>[8x]MSLIVITGASSGLGAELAKLYDAEGKATYLTGRSESKLSTVTN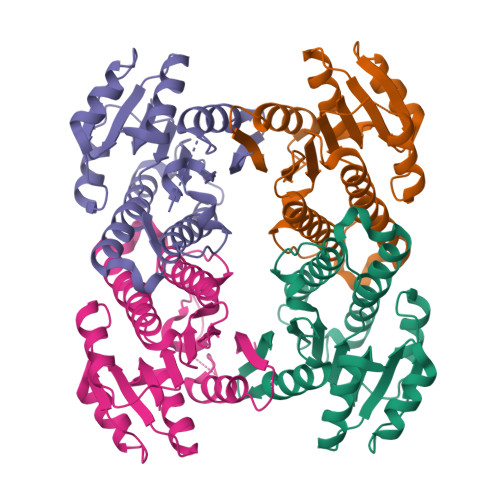CLSNNVGYRARDLASHQEVEQLFEQLDSIPSTVVHSAGSGYFGLLQEQDPEQIQTLIENNLSSAINVLRELVKRYKDQPVNVVMIMSTAAQQPKAQESTYCAVKWAVKGLIESVRLELKGKPMKIIAVYPGGMATEFWETSGKSLDTSSFMSAEDAALMIHGALANIGNGYVSDITVNREGHHHHHH Gloeobacter violaceus proton-gated ion channel (GLIC), a prokaryotic model of pLGICs, is particularly well-suited to stabilize preactive states under suboptimal activating conditions modulated by pH. The GLIC homomer consists of five subunits, each with an ECD and TMD. GLIC is activated by the protonation of a series of titratable residues in the ECD, leading to counterclockwise rotation and contraction of the ECD. Therefore, we established a data processing strategy involving symmetry expansion, backtracking particles, supervised particle reorientation, and 3D reconstruction to resolve high-resolution maps of various asymmetric intermediate states of nanodisc-reconstituted GLIC at pH 4.0, which provide comprehensive understanding of activation mechanism of GLIC.

Further using our data processing approach, six high-resolution asymmetric maps with configurations of iiiio (or i4o1), iiioo (or i3o2), iiooo (or i2o3), ioooo (or i1o4), iioio, and ioioo were reconstructed without imposing symmetry with resolutions ranging from 3.08 to 3.45 Å. Subsequently, when subunit D adopts o conformation (i3o2), I16′ of subunit E(o) and L17′ of subunit D(o) undergo radial displacements compared to i4o1 state. This is likely driven by the combined influence of subunit D activation and conformational drive exerted by principal subunit E(o). However, this scenario changes when subunit D is activated and adopts the o conformation (i3o2). In this state, L17′ in the M2 helix of subunit D(o) is already under steric strain from I16′ of subunit E(o). This strain is further amplified by the activation of subunit D. The combined effect of these forces causes radial displacement of L17′, resulting in outward displacement of the M2 helix in subunit D(o) along with I16′ in subunit E(o) as indicated by the expanded pore. The changes in pore radius of i4o1 compared to i5 state is indistinguishable, whereas the pore gradually expands from i3o2 state onward and maximum expansion occurs in the o5 state. In the i4o1, i3o2, and i2o3 states, the pore radii at I9′ are narrower than the hydrated Na+ ion (2.76 Å), indicating nonconductive states.

>[5x]VSPPPPIADEPLTVNTGIYLIECYSLDDKAETFKVNAFLSLSWKDRRLAFDPVRSGVRVKTYEPEAIWIPEIRFVNVENARDADVVDISVSPDGTVQYLERFSARVLSPLDFRRYPFDSQTLHIYLIVRSVDTRNIVLAVDLEKVGKNDDVFLTGWDIESFTAVVKPANFALEDRLESKLDYQLRISRQYFSYIPNIILPMLFILFISWTAFWSTSYEANVTLVVSTLIAHIAFNILVETNLPKTPYMTYTGAIIFMIYLFYFVAVIEVTVQHYLKVESQPARAASITRASRIAFPVVFLLANIILAFLFFG>MAGSGKFFVGGNWKCNGTKDSIAKLISDLNSATLEADVDVVVSPPFVYIDQVKSSLTDRID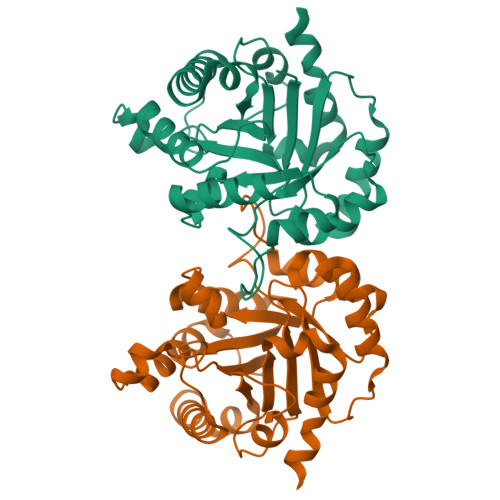ISGQNSWVGKGGAFTGEISVEQLKDLGCKWVILGHSERRHVIGEKDEFIGKKAAYALSEGLGVIACIGEKLEEREAGKTFDVCFAQLKAFADAVPSWDNIVVAYEPVWAIGTGKVASPQQAQEVHVAVRGWLKKNVSEEVASKTRIIYGGSVNGGNSAELAKEEDIDGFLVGGASLKGPEFATIVNSVTSKKVAA[2x]>[2x]MAAAPLKV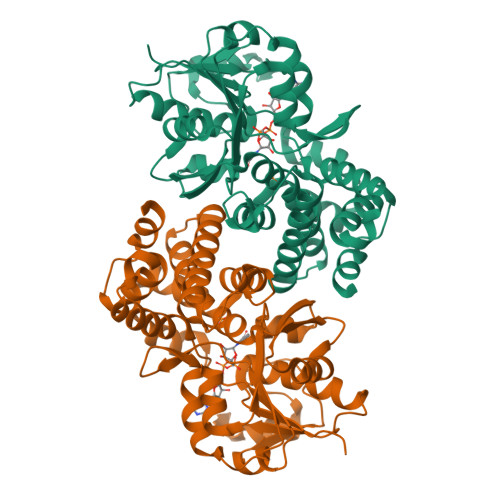CIVGSGNWGSAVAKIIGNNVKKLQKFASTVKMWVFEETVNGRKLTDIINNDHENVKYLPGHKLPENVVAMSNLSEAVQDADLLVFVIPHQFIHRICDEITGRVPKKALGITLIKGIDEGPEGLKLISDIIREKMGIDISVLMGANIANEVAAEKFCETTIGSKVMENGLLFKELLQTPNFRITVVDDADTVELCGALKNIVAVGAGFCDGLRCGDNTKAAVIRLGLMEMIAFARIFCKGQVSTATFLESCGVADLITTCYGGRNRRVAEAFARTGKTIEELEKEMLNGQKLQGPQTSAEVYRILKQKGLLDKFPLFTAVYQICYESRPVQEMLSCLQSHPE> GAIKIEIPPDAPPQAVADAAVAALRAADPGAARRRVTFDVTGPDAARVQALADAVVAALEREGFKLEKKEENTDAAGNAGAKYEGEGGLVLNVKQGPE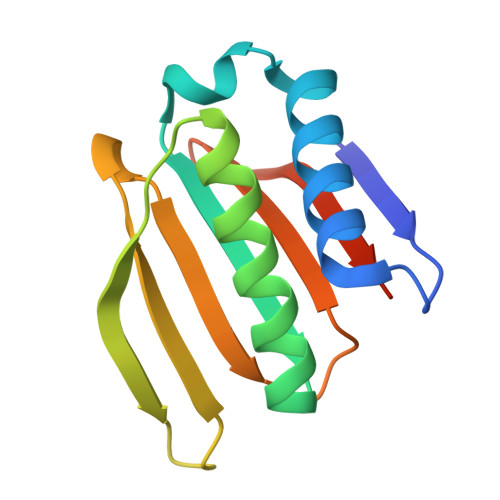ALTLKITVDGRTIVEIVRLEHHHHHH>GMATYNYPEFGAGLWHFANYIDRYAVDGYGPALSTIDQINAAKEVGELSYVDLPYPFTPGVTLSEVKDALKDAGLKAIGITPEIYLQKWSRGAFTNPDPAARAAAFELMHESAGIVRELGANYVKVWPGQDGWDYPFQVSHKNLWKLAVDGMRDLAGANPDVKFAIEYKPREPRVKMTWDSAARTLLGIEDIGLDNVGVLLDFGHALYGGESPADSAQLIIDRGRLFGMDVNDNLRGWDDDLVVGTVHMTEIFEFF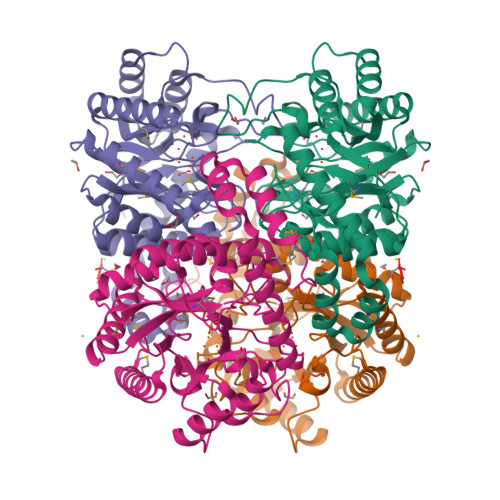YVLKINNWQGVWQLDQFPFRENHVEAAQLSIRFLKHIYRALDKLDIPALQAAQEAQNPLQAQRIVQDALLSSITVSE[2x]>[6x]MTKLLDGKVAFITGSASGIGLEIAKKFAQEGAKVVISDMNAEKCQETANSLKEQGFDALSAPCDVTDEDAYKQAIELTQKTFGTVDILINNAGFQHVAPIEEFPTAVFQKLVQVMLTGAFIGIKHVLPIMKAQKYGRIINMASINGLIGFAGKAGYNSAKHGVIGLTKVAALECARDGITVNALCPGYVDTPLVRGQIADLAKTRNVSLDSALEDVILAMVPQKRLLSVEEIA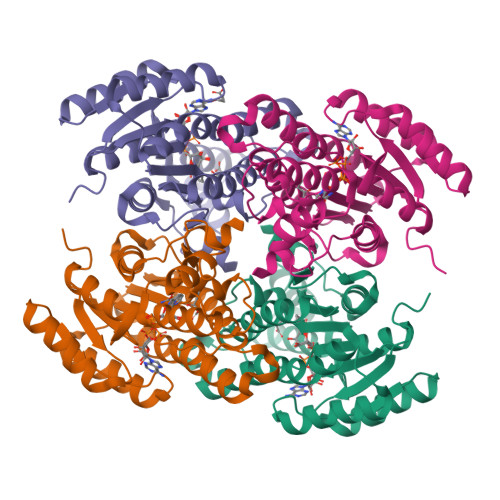DYAIFLASSKAGGVTGQAVVMDGGYTAQ> QSISPNELGLTSAQDDGPLGNEKPNYFLNFRTMNVDIFTVSHTKVDNIFGRAWYVASHDFNNGDTWRQKLTFPKEGHGMLSQFFAYFTGEINIHILYMAEQGFLRVAHTYDTEDNRKTFLSSNGVITIPAGEQMTLSVPFYSNKPLRTVRHDSALGFLMCRPMMHGTTRTTAEVYISLRCPNFFFPVPAPKPTGSRAA;> TKYKWTRTKVDIAEGPGTMNMANVLSTTGAQSVALVGERAFYDPRTAGSKSRFDDMIKIAQLFSVMSDNTTPSSSSGIDKYGYFDWAATVAPQNMVHRNVVTLDQFPNLNLFMNTYSYFRGSLIIRLSIYASTFNRGRLRMGFFPNCTHDTQLELDNAIYTICDIGSDNSFELTIPYSFSTWMRKTHGHQLGLFQVEVLNRLTYNSSSPNKVHCIVQGRLGDDAKFFCPTGSLVSFQ;> LSNVETEANNIISGNEVGGEIITKVADDASNLLGPNSFATTAQPENKDVVQATTTVNTTN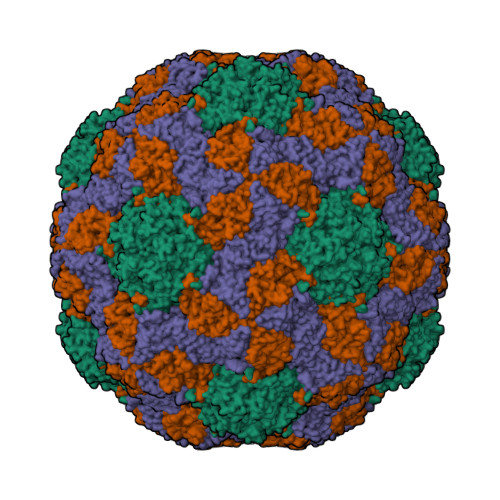LTQHPSAPTIPFTPDFRNVDNFHSMAYDITTGDKNPSKLIRLDTASWQTSYSRQYKITTVELPKSFWDDTRKPAYGQAKYFAAVRCGFHFQVQVNVNQGTAGSALVVYEPKPVIDSRQYLEFGSLTNLPHVLMNLAETTQADLCIPYVADTNYVKTDSSDLGQLRVYVWTPLSVPTGASNEVDVTVMGSLLQLDFQNPRPYGE Alcohol dehydrogenases (ADHs), also known as ketoreductases (KREDs), are of great industrial interest primarily due to their ability to perform an asymmetric reduction of aldehydes and ketones. Switching the cofactor preference of NADP-dependent enzymes to NAD is of particular interest due to the lower cost and higher stability of NAD, and the higher efficiency of cell-free NAD recycling systems, for which low-cost co-substrates are available. We crystallized CBADHS and TBADHS1 in order to elucidate the structural basis for the observed reversal of cofactor preference. In both cases, the size of the cofactor-binding pocket is reduced due to the substitution of residues 198 and 199 by others with bulkier side chains, which sterically prevents the binding of the 2′ phosphate of NADP.

We performed full combinatorial saturation mutagenesis of all four target residues of CBADH (G198, S199, R200, and Y218) replacing each codon with NNN to yield a library (CBADHLib) of 16.8 million unique genetic variants encoding 160,000 unique protein variants. Growth was observed in three of the variant pools so these were each subcultured under the same conditions once, then plasmid DNA was extracted and sequenced, revealing the presence of the same CBADH variant in each case (CBADHS) with G198D, S199Y, and Y218P substitutions. Unlike the parent enzyme CBADHWT, purified CBADHS was unable to oxidize isopropanol using oxidized NADP (NADP+) as the cofactor, but could do so with NAD+ (Km = 17.49 mM, kcat = 333 min−1 and kcat/Km = 316.67 M−1 s−1). The resulting maps showed clear density for NAD+ in the case of CBADHS, but only partial occupancy for TBADHS1. In the case of CBADHS, this effect is further enhanced by the presence of an aspartate residue at position 198, which would also prevent NADP binding through electrostatic repulsion between the side-chain carboxylate group and the 2′ phosphate of NADP. Interestingly, NAD-dependent mouse class II alcohol dehydrogenase (ADH2), which is distantly related to CBADH, contains D227 and P247 which are equivalent positions to 198 and 218 in CBADH. CBADHS was not among the 567 variants proposed by CSR-SALAD. However, only NAD-dependent CBADHS could support acetone-dependent anaerobic growth of ALPS cells, which lack either intact transhydrogenase gene.

>[4x]MKGFAMLGINKLGWIEKERPVAGSYDAIVRPLAVSPCTSDIHTVFEGALGDRKNMILGHEAVGEVVEVGSEVKDFKPGDRVIVPCTTPDWRSLEVQAGFQQHSNGMLAGWKFSNFKDGVFGEYFHVNDADMNLAILPKDMPLENAVMITDMMTTGFHGAELADIQMGSSVVVIGIGAVGLMGIAGAKLRGAGRIIGVDYRPICVEAAKFYGATDILNPKNGHIVDQVMKLTNGKGVDRVIMAGGGSETLSQAVSMVKPGGIISNINYHGSGDALLIPRVEWGCGMAHKTIKGGLCPGGRLRAEMLRDMVVYNRVDLSKLVTHVYHGFDHIEEALLLMKDKPKDLIKAVVILHHHH>GMSKIFNEELAVIEAAAIAYLTAFNRADIPAVIATYTDDGVLMGPGRPAAVGKDELAEVYLSVFETVGFDMAYEIKEVVQTSAD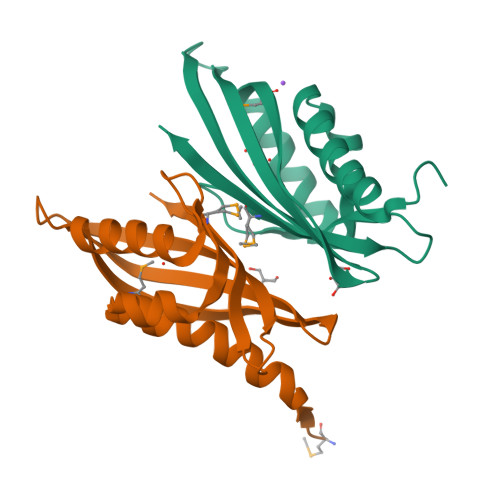WAFVRSATEGTETNKATGVVTPAAYQELFLLRKSATGSWQTARYCTSKISP[4x]Here we use structural and biophysical approaches combined with molecular dynamics to study transport by Arabidopsis thaliana LAX3, which is essential for plant root formation. Structurally, LAX3 consists of a bundle and a scaffold domain. The ligand-binding site is sandwiched between these domains with two histidines occupying positions analogous to the sodium-binding sites in distantly related sodium:neurotransmitter transporters. This architecture suggests that these histidines couple transport to the proton motive force.

In the presence of IAA, well-defined density is seen in the binding pocket. In this IAA-bound state, access from the cytosol is constricted by a thin gate composed of His189 and Arg192 on the M4–M5 loop, Val249 and Glu252 on M6b, and Phe326 and Thr329 on M8. This architecture defines the IAA-bound structure as an inward semi-occluded bound conformational state in which the ligand binding site is still water accessible. IAA is bound with its carboxylate group in this polar region pointing towards the apoplast side and interacting with the unwound portions of M1 and M6. The carboxylate interacts with Gln60(M1), Tyr242(M6), His247(M6) and the backbone amide of Ala59(M1). The indole ring of IAA is situated in the hydrophobic region defined by Phe143(M3), Leu144(M3), Val249(M6), Phe326(M8), Ala327(M8) and Pro330(M8). Here, the indole ring occupies the space between M1 and scaffold helices M3 and M8, with hydrogen bonding to the side-chain amide and main-chain carbonyl of Asn56(M1). His247 is of particular interest because it engages directly with the carboxyl group of IAA. MD simulations illustrate the dynamics of IAA within the binding site in the inward semi-occluded state. Notably, they show that IAA can flip 180° and interact with Arg192, an interaction that requires dynamic changes to the M5 helix.

> MGSVYDAWFSCASNQVAQVLLTLPYSFSQLGMMSGILFQLFYGLMGSWTAYLISVLYVEYRTRKEREKFDFRNHVIQWFEVLDGLLGKHWRNLGLIFNCTFLLFGSVIQLIACASNIYYINDKLDKRTWTYIFGACCATTVFIPSFHNYRIWSFLGLAMTTYTSWYLTIASLLHGQAEDVKHSGPTTMVLYFTGATNILYTFGGHAVTVEIMHAMWKPQKFKAIYLLATIYVLTLTLPSASAVYWAFGDKLLTHSNALSLLPKTGFRDTAVILMLIHQFITFGFASTPLYFVWEKLIGVHETKSMFKRAMARLPVVVPIWFLAIIFPFFGPINSAVGSLLVSFTVYIIPALAHMLTFAPAPSRENAVERPPRVVGGWMGTYCINIFVVVWVFVVGFGFGGWASMVNFVRQIDTFGLFTKCYQCPPHKPGENLYFQ>MSTNKVNKERTFLAVKPDGVARGLVGEIIARYEKKGFVLVGLKQLVPTKDLAESHYAEHKERPFFGGLVSFITSGPVVAMVFEGKGVVASARLMIGVTNPLASAPGSIRGDFGVDVGRNIIGGSDSV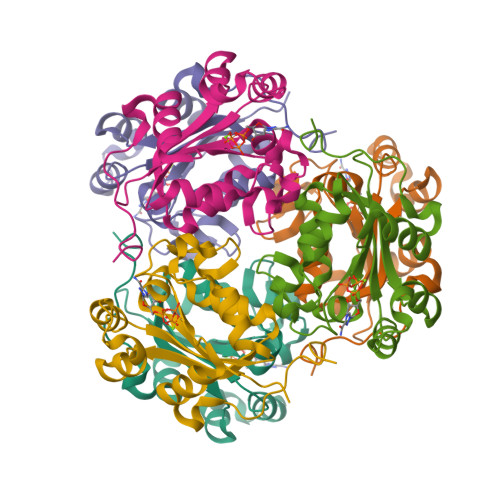ESANREIALWFKPEELLTEVKPNPNLYE[3x]> SHMSLIRGVVVSKQLVYDPTGTK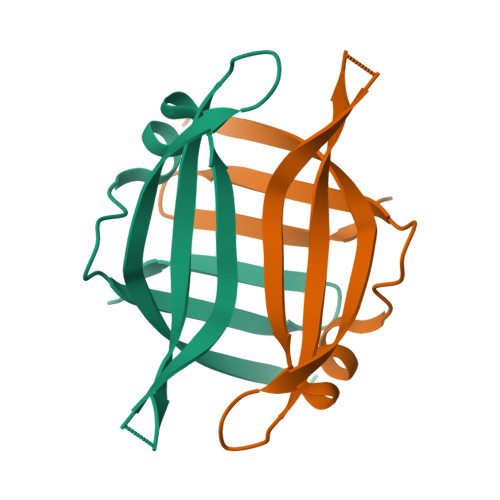YVKIDVVEEKELPGPVAAFSAQDEQAAQLMREVMPLVTQIVRSLPFGGGKITVPRITLWLTEEEEEVFGDIDVGDVIEINIENGAITIKPES>[4x]MSLDKIRYGIMSTAQIVPRFVAGLRESAQAEVRGIASRRLENAQKMAKELAIPVAYGSYEELCKDETIDIIYIPTYNQGHYSAAKLALSQGKPVLLEKPFTLNAAEAEELFAIAQEQGVFLMEAQKSVFLPITQKVKATIQEGGLGEILWVQSVTAYPNV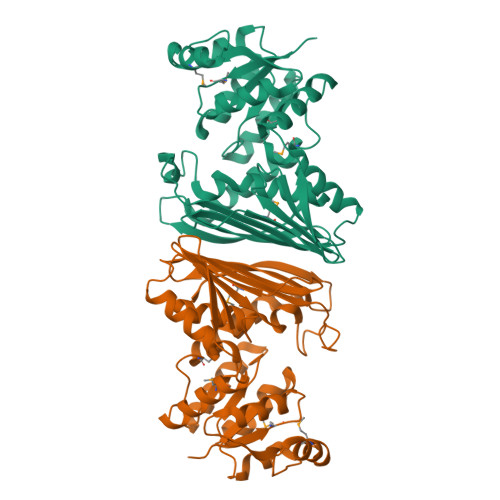DHIPWFYSREAGGGALHGSGSYPLQYLQYVLGKEIQEVTGTATYQQGATDSQCNLALKFAEGTLGNIFINVGLKIPSEMTICGTKGQIVIPNFWKTDCAYYTDAQGNTVKWSEQFTSEFTYEINHVNQCLQDKKLTSPVMTKELTIATVKIVESFYQEWFDNEGHHHHHH3-[4-(aminomethyl)phenyl]-6-[[1-[[2-chloranyl-4-(1,2,4-oxadiazol-3-yl)phenyl]methyl]-4-oxidanyl-piperidin-4-yl]methyl]-2-methyl-pyrazolo[4,3-d]pyrimidin-7-one | C28 H29 Cl N8 O3 | 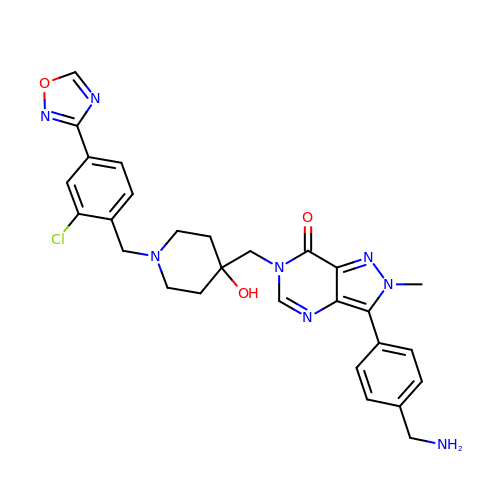SUBLUDSEMODLLX-UHFFFAOYSA-N> EPLAAGAVILRRFAFNAAEQLIRDINDVASQSPFRQMVTPGGYTMSVAMTNCGHLGWTTHRQGYLYSPIDPQTNKPWPAMPQSFHNLCQRAATAAGYPDFQPDACLINRYAPGA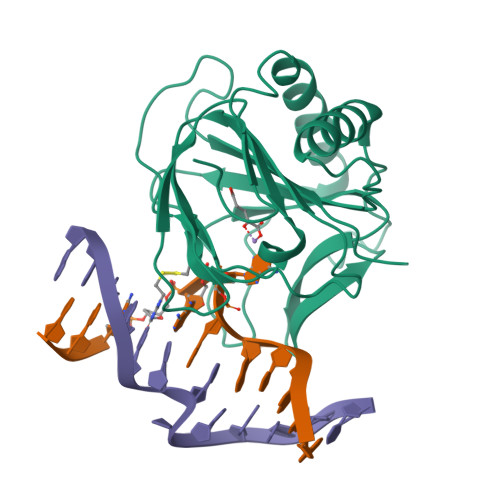KLCLHQDKDEPDLRAPIVSVSLGLPAIFQFGGLKRNDPLKRLLLEHGDVVVWGGESRLFYHGIQPLKAGFHPLTIDCRYNLTFRQAGK>[2x]NDFKNHQLPLARIKKIMKAD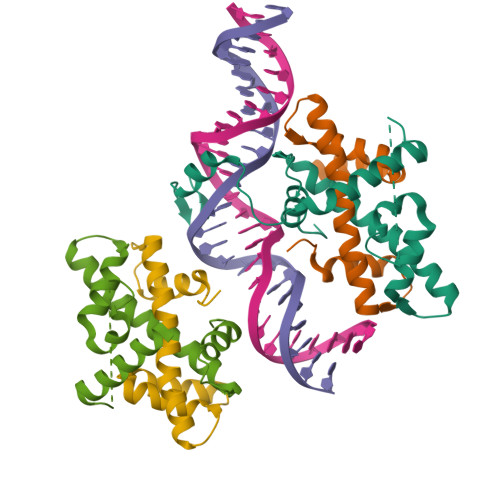EDVRMISAEAPILFAKACELFILELTIRSWLHAEENKRRTLQKNDIAAAITRTDIFDFLVDIVPRGSGSGSGSGSGSDPASQMITVTQLSPMDREARVLRYREKRKTRKFEKTIRYASRKAYAEIRPRVNGRFAKREIEAEEQGF;>STREQDRFLPIANVSRIMKKALPANAKISKDAKETVQECVSEFISFITGEASDKCQREKRKTINGDDLLWAMTTLGFEDYVEPLKVYLQKYREVEGEKTTTAG[2x]> GSHMLKGQEFAPSHQQVYAPLRADGDKPRAHLTVVRQTPTQHFKNQFPALHWEHELGLAFTKNRMNYTNKFLLIPESGDYFIYSQVTFRGMTSESSEIRQAGRPNKPDSITVVITKVTDSYPEPTQLLMGTKSVSEVGSNWFQPIYLGAMFSLQEGDKLMVNVSDISLVDYTKEDKTFFGAFLL;> RSVAETPTYPWRDAETGERLVCAQCPPGTFVQRPCRRDSPTTCGPCPPRHYTQFWNYLERCRYCNVLCGEREEEARACHATHNRACRCRTGFFAHAGFCLEHASCPPGAGVIAPGTPSQN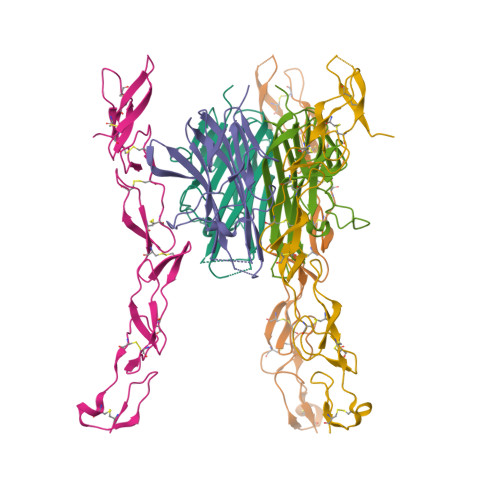TQCQPCPPGTFSASSSSSEQCQPHRNCTALGLALNVPGSSSHDTLCTSTGHHHHHH>FKRIVQRIKDFLR[2x]

The hLL-3717–29 fragment was suggested to serve as the active core of the AMP, showing a different spectrum of antibacterial activity as compared to the full-length protein and other fragments, including being the shortest LL-37 fragment retaining anti-viral activity. Here we demonstrate that the active core peptide of hLL-37, containing residues 17–19 (hLL-3717–29), formed supra-helical highly stable fibrils that interact with bacterial cells. Rather, the fibrillar assembly of LL-3717–29 was comprised of associating four-helix bundles, each stabilized by a closely packed hydrophobic core. To conclude, the atomic structures of human and primate antibacterial LL-3717-29 showed a functional supramolecular nanostructure of densely packed amphipathic helices.

Our determination of the crystal structure of hLL-3717–29 at 1.35 Å resolution, revealed self-assembly of amphipathic helices into a densely packed and elongated hexameric structure forming a central pore. There were two helices in the asymmetric unit of the crystal, with 67% of their individual solvent accessible surface areas buried within the assembly, indicating compact packing. The structure of LL-3717–29 lacked amyloid continuous sheets with individual molecules stacked perpendicular to the fibril axis, and correspondingly did not bind the amyloid indicator dye Thioflavin T, in contrast to the cross-α amyloid fibrils of PSMα322. Arginine residues are lined on the surface of the bundles, with side chains extending outwards, providing an overall highly positively charged molecular electrical potential surface. The interfaces between bundles comprises a network of polar interactions, including potential salt bridges between Asp26 and Arg23/Arg29 from two adjacent helices, and between Lys25 and the C-terminus of an adjacent helix. The fibrillar assembly in the crystal structure created alternating hydrophobic and polar (positively charged) zigzagged belts on its surface, suggesting interactions with and disruption of negatively charged lipid bilayers, such as bacterial membranes. The overall stable assembly of LL-3717–29, which includes a network of polar interactions and hydrophobic packing, corresponded with the thermostability of the fibrils, as visualized by electron micrographs after heating to 60 or 80 °C. Alanine substitution of Ile24, the most buried residue within the core of the four-helix bundle, abolished antibacterial activity against M. luteus and against S. hominis. In the hLL-3717-29 structure, the lysine residues are almost perpendicular to the cross-section of the pore.>[2x]MAQEDVTAVATNGAGPVETHLVFTEFKQMLLVEAQKVGDAVTFYKSAFGAIESGHSLYPKRKLDQELPHVLSSELNLA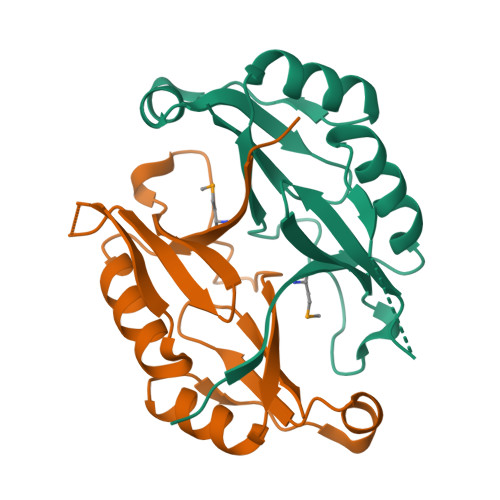GSSFVVCDVSSLPGFSTAKSEGSGVTFLLGTKDAEAAVAKAVDAGAVKVEVTEAEVELGFKGKVTDPFGVTWIFAEKKTVITDENKEV> GPKQKIVIKVSMPCEKSRSKAMKLVVMASGVSSVEVTGDGKDRLQVVGDGVDAACLVTCLRKKIGHAELVQVEEVKEK;> GPETGNKYIEKRAIDLSRERDPNFFDNADIPVPECFW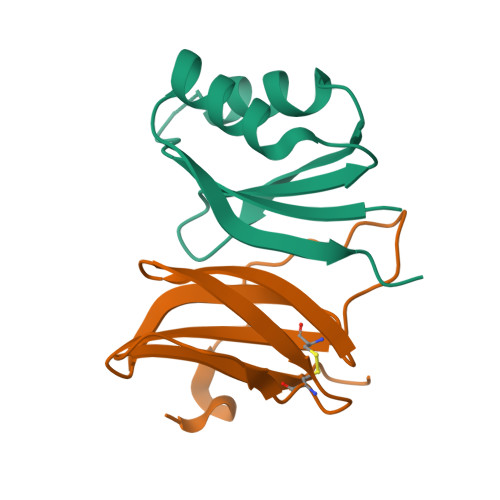FMFKNNVRQDAGTCYSSWKMDKKVGPNWVHIKSDDNCNLSGDFPPGWIVLGKKRPGF>[2x]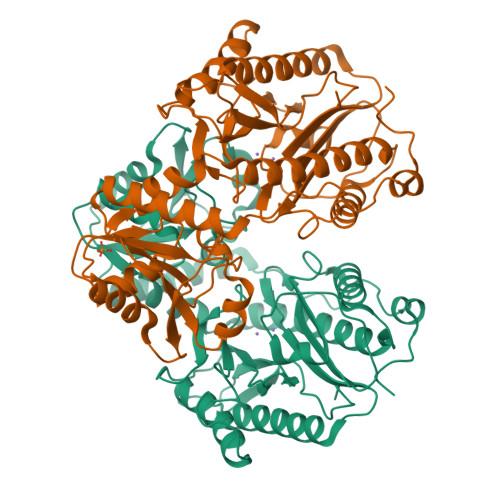GSSTQIGGMSLDQARTQLAPWTQRAAPIGADEYQQRIERARVLMRAQGVDALLIGAGTSLRYFSGVPWGASERLVALLLTTEGDPVLICPAFEEGSLDAVLQLPVRKRLWEEHEDPYALVVQAMDEQHAHALALDPGIAFAVHTGLRAHLGTAIRDAGAIIDGCRMCKSPAELALMQQACDMTLLVQRLAAGIAHEGIGTDQLVRFIDEAHRALGADNGSTFCIVQFGHATAFPHGIPGVQHLRAGELVLIDTGCTVQGYHSDITRTWIYGTPSDAQQRIWELELAAQAAAFAAVRPGVACEAVDQAARAVLQAAGLGPDYRLPGLPHRTGHGCGLAIHEAPYLVRGNRQPLQPGMCASNEPMIVVPGAFGVRLEDHFYVTDTGAQWFTPPSVAIDQPFA> AQIHVLVLHGPNLNLLGRREPDHYGRTTLAEIDARLKTEAEGRGWLLHSLQSNAEHI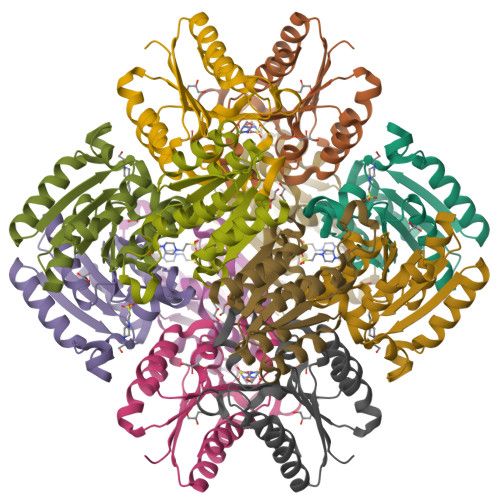LVDAVQQAPTQGVTHIVLNPAAFTHTSVALRDALAAVAIPFIEVHLSNIHAREPFRRHSYFSDIASGLITGLGAEGYSLALDAIARRF>GAMAGKSSLFKVILLGDGGV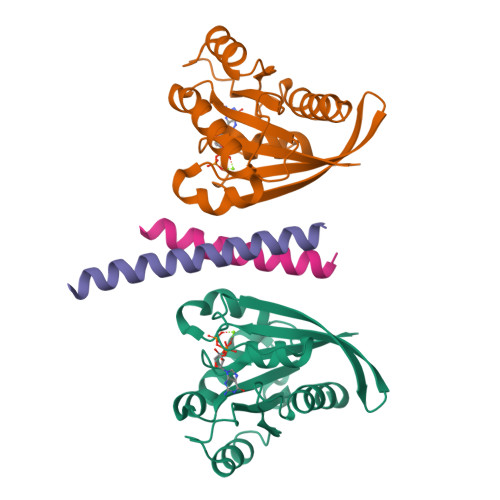GKSSLMNRYVTNKFDTQLFHTIGVEFLNKDLEVDGHFVTMQIWDTAGLERFRSLRTPFYRGSDCCLLTFSVDDSQSFQNLSNWKKEFIYYADVKEPESFPFVILGNKIDISERQVSTEEAQAWCRDNGDYPYFETSAKDATNVAAAFEEAVRRVLATEDRSDHLIQTDTVNLHRKPKPSSSCC[2x];>MDDLAQTKAIKDQLQKYIRELEQANDDLERAKRATIMSLEDFEQRLNQAIERNAFLESELDEKENLLESVQR[2x]>EEVRQFRRLFAQLAGDDMEVSATELMNILNKVVTRHPDLKTDGFGIDTCRSMVAVM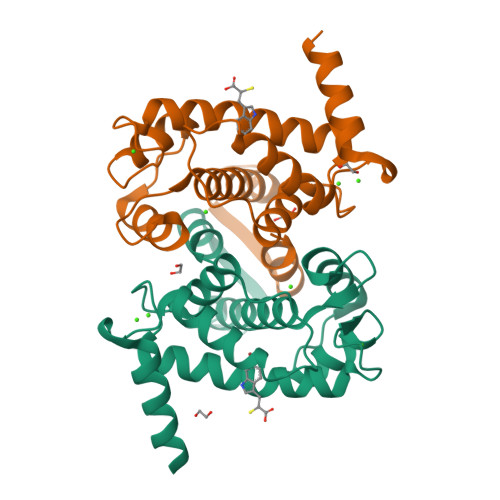DSDTTGKLGFEEFKYLWNNIKRWQAIYKQFDTDRSGTICSSELPGAFEAAGFHLNEHLYNMIIRRYSDESGNMDFDNFISCLVRLDAMFRAFKSLDKDGTGQIQVNIQEWLQLTMYS[2x]N-(1-acetyl-1H-indol-3-yl)-N-(5-hydroxy-2-methylphenyl)acetamide 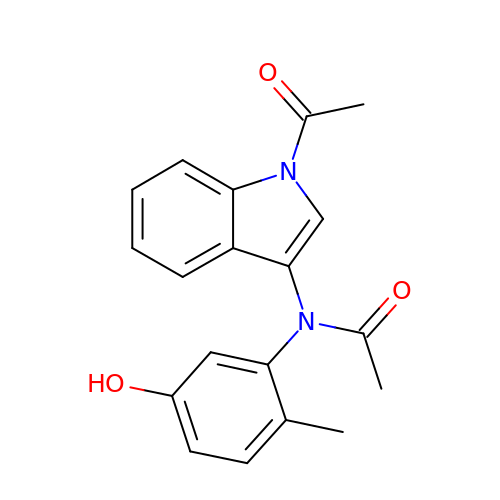| C19 H18 N2 O3 | NXETYAFZIDRMKK-UHFFFAOYSA-N>GKITFYEDRGFQGRHYECSSDHSNLQPYLGRCNSVRVDSGCWMIYEQPNYLGPQYFLRRGDYPDYQQWMGLNDSIRSCRLIPHAGSHRLRLYEREDYRGQMIEITEDCSSLQDRFHFNEIHSLNVLEGSWVLYELPNYRGRQYLLRPG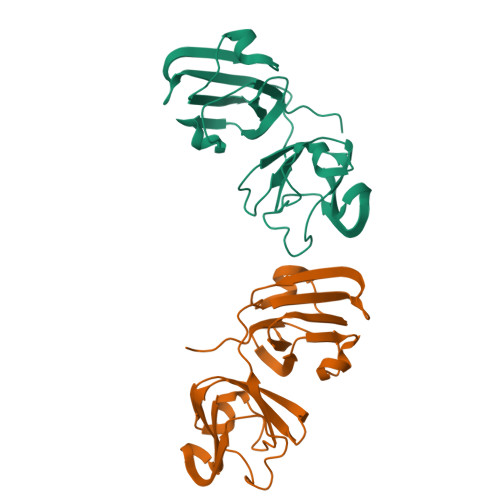EYRRYHDWGAMNAKVGSLRRVIDIY[2x]> GPLGSLFRSLVGTSRAIQQVRQMMQQVADTDASVLILGESGTGKEVVARNLHYHSKRREGPFVPVNCGAIPAELLES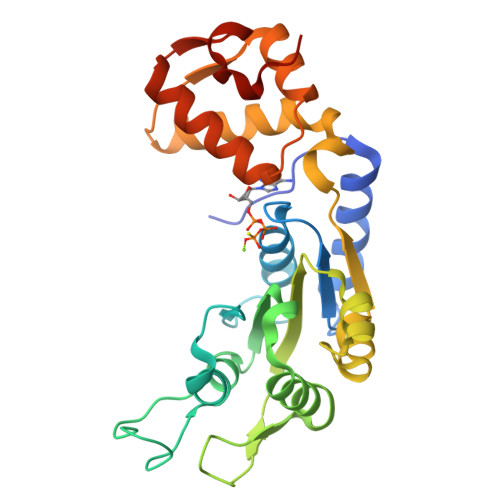ELFGHEKGAFTGAITSRAGRFELANGGTLFLDEIGDMPLPMQVKLLRVLQERTFERVGSNKTQNVDVRIIAATAKNLEKMIEDGTFREDLYYRLNVFPIEMAPLRERVEDIALLLNELISRMEHEKRGSIRFNSAAIMSLCRHDWPGNVRELANLVERLAIMHPYGVIGVGELPKKFRHVDDEDEQ AMPylation (or adenylylation) is the transfer of AMP from ATP to a Tyr or Thr/Ser residue in target proteins. Interestingly, in eukaryotic genomes only one FIC-domain containing protein has been identified to date, HYPE or FICD, and it is strongly conserved from C. elegans to humans. Here we describe the first crystal structure of a eukaryotic HYPE encompassing the two TPR-motifs, an α-helical linker, and the FIC domain of the human protein. We demonstrate that HYPE forms stable dimers with structurally and functionally integrated FIC-domains and with TPR-motifs exposed for protein-protein interactions.

In addition to apo structures of HYPE variants, we have also obtained structures with the ATP cofactor bound to an E234G variant and with ADP bound to either the HYPE E234G variant or to wild-type protein. The adenosine moiety of the ATP and ADP locks into a hydrophobic pocket formed between α3, αpost A and the flap loop; the side chain residues forming this pocket are Val360 (α3), Leu403 (αpost A), and Val316 (flap). The GNG anion hole (residues 368–370) accommodates the α-phosphate of the nucleotide, mainly through direct hydrogen bonds to the polypeptide backbone. A Mg2+ ion is visible in the E234G variant of HYPE; it bridges the α- and β-phosphates and is coordinated by the conserved Asp367 side chain. The position of clearly visible α- and β-phosphates in all three structures is the same, with the α-phosphate present in an orientation compatible with the AMPylation reaction. Measurements of binding of a range of ligands to the E234G variant (172–434) using thermal shift analysis excluded phosphocholine as a possible cofactor (utilized by some FIC-domain proteins such as AnkX) (no shift in Tm, data not shown) and showed similar binding of ATP and guanosine-5'-triphosphate, and a less strong binding of cytidine triphosphate and uridine triphosphate. Interestingly, binding of ADP was stronger than that of ATP. A possible reason could be that ATP adopts a less favorable conformation within the binding pocket compared to free ATP, a constraint that would not apply to ADP. The measurement of the dissociation constant (KD) of ADP binding to the E234G variant determined by isothermal titration calorimetry (ITC) was 160 nM.

>GKLEARAALNQALEMKRQGKREKAQKLFMHALKMDPDFVDALTEFGIFSEEDKDIIQADYLYTRALTISPYHEKALVNRDRTLPLVEEIDQRYFSIIDSKVKKVMSIPKGNSALRRVMEETYYHHIYHTVAIGGNTLTLSEIRHILETRYAVPGKSLEEQNEVIGMHAAMKYINTTLVSRIGSVTISDVLEIHRRVLGYVDPVEAGRFRTTQVLVGHHIPPHPQDVEKQMQEFVQWLNSEEAMNLHPVEFAALAHYKLVYIHPFIDGNGRTSRLLMNLILMQAGYPPITIRKEQRSDYYHVLEAANEGDVRPFIRFIAKCTETTLDTLLFATTEYSVALPEAQP[2x]The crystal structures of the proteins encoded by the YP_749275.1 and YP_001095227.1 genes from Shewanella frigidimarina and S. loihica, respectively, have been determined at 1.8 and 2.25 Å resolution, respectively. These proteins are members of a novel family of bacterial proteins that adopt the α/β SpoIIAA-like fold found in STAS and CRAL-TRIO domains.

The YP_749275.1 gene from Shewanella frigidimarina encodes a protein of unknown function with a molecular weight of 14 502 Da (residues 1–126) and a calculated isoelectric point of 4.9. The final model of YP_749275.1 consists of a protein dimer (residues 2–126 for chain A and residues 3–79 and 82–126 for chain B), six ethylene glycols and 224 water molecules in the asymmetric unit. In the ‘closed’ structure (YP_749275.1), the helices partially unfold and rearrange, occluding the cavity and decreasing the solvent-exposed hydrophobic surface. In contrast, in YP_749275.1, α-helices α2 and α3 are substantially shortened (from four and five to one and 2–3 helical turns, respectively) and α3 is rotated by ∼90° from its orientation in YP_001095227.1. In addition, α3 shifts by ∼5 Å towards α2 and thus eliminates the cavity. Residues from α2 (Trp71, Leu74 and Leu78) and α3 [Trp98, Val102 (Ile in YP_749275.1), Trp105 and Phe106], which are exposed to solvent in YP_001095227.1, relocate into the protein interior. For example, in the ‘closed’ state, Trp71 is buried from the solvent and participates in multiple van der Waals interactions with surrounding aromatic and aliphatic residues (Leu8, Leu29, Tyr34, Leu74 and Trp65), while His6 and His31 face the solvent and are not involved in any stabilizing hydrogen bonds. Arg14 of one subunit hydrogen bonds to Asp33 of the other subunit, which is likely to provide some stability and specificity to the dimer formation (YP_749275.1). The lack of conservation of this serine in YP_749275.1 indicates a possible loss of functional similarity to SpoIIAA.

>[2x]GMDMKKHGLSIGINRIESVFFVTLKAIGTLTHEDYLVITPMLEGALSQVDQPKVSLFLDATELDGWDLRAAWDDLKLGLKHKSEFERVAILGNKDWQEWAAKIGSWFIAGEIKYFEDEDDALKWLRY> MASSSTPRFRVYSKYLFLTYPQCTLEPQYAL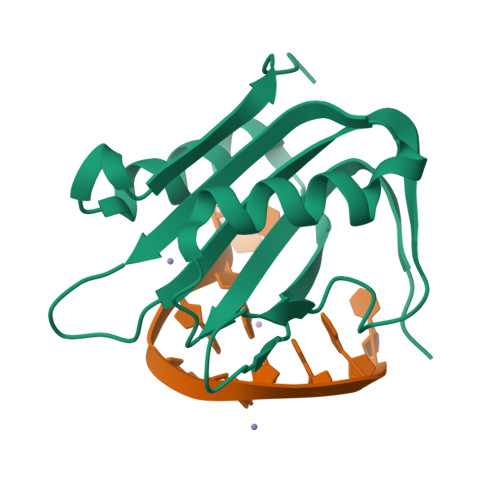DSLRTLLNKYEPLYIAAVRELHEDGSPHLHVLVQNKLRASITNPNALNLRMDTSPFSIFHPNIQAAKDCNQVRDFITKEVDSDVNTAEWGTFVAVSTPGRKDRDAD>GAMASNTNLIV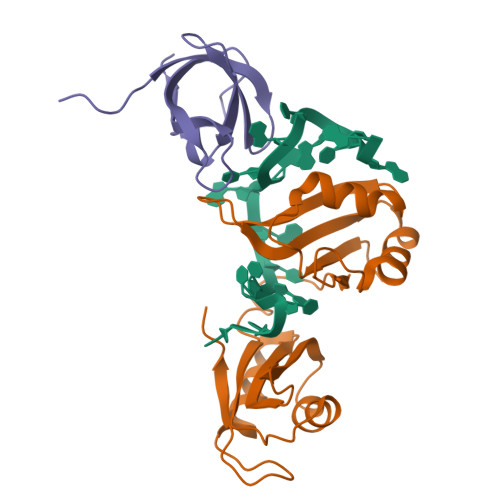NYLPQDMTDRELYALFRAIGPINTCRIMRDYKTGYSFGYAFVDFTSEMDSQRAIKVLNGITVRNKRLKVSYARPGGESIKDTNLYVTNLPRTITDDQLDTIFGKYGSIVQKNILRDKLTGRPRGVAFVRYNKREEAQEAISALNNVIPEGGSQPLSVRLAEEHGK[2x];>[2x]GAMATRETGIIEKLLHSYGFIQCCERQARLFFHFSQFSGNIDHLKIGDPVEFEMTYDRRTGKPIASQVSKIA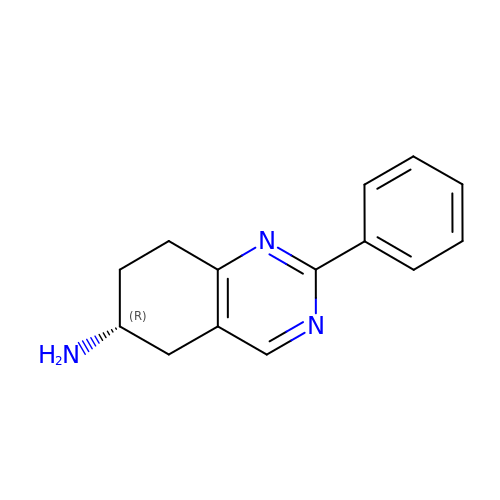(6~{R})-2-phenyl-5,6,7,8-tetrahydroquinazolin-6-amine | C14 H15 N3 | DBOFAIZAMCFPNL-GFCCVEGCSA-N>SKINVNVENVSGVQGFLFHTDGKESYGYRAFINGVEIGIKDIE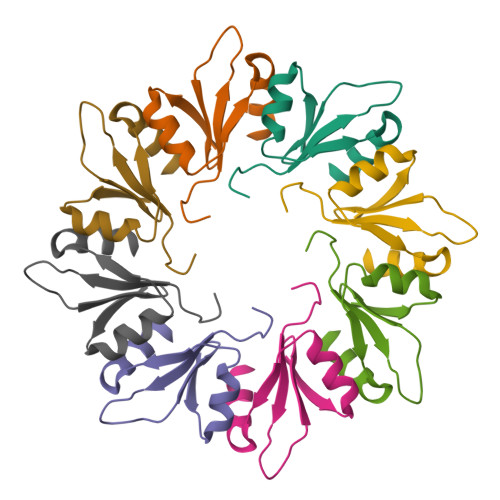TVQGFQQIIPSINISKSDVEAIEKAMKK[2x]>[2x]MAHHHHHHMVSWFKKIFKKEEKES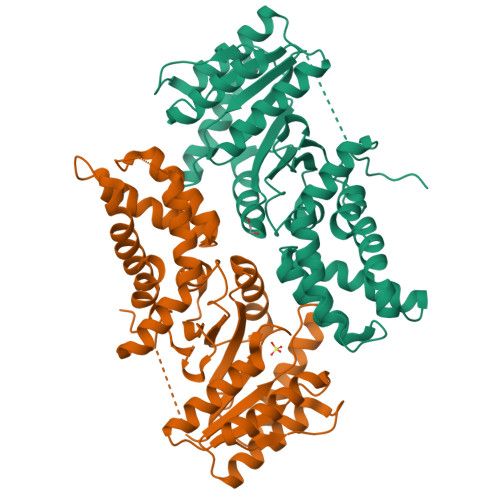LDKGLEKSSQSFFDKVSRAVVGKSKVDDEVLDDLEEVLIASDVGVETTVKIIRRIEERVARDKYVNVAELNNILREEISGLLLENPHAGTQNIDKTKKPYVIMVVGVNGVGKTTTIGKLAHQFKSEGLKVVLGAADTFRAAAVDQLVIWSERVGVPIVKQAMGSDPASVAFDTVQSAVSQDADVVIIDTAGRLHNKVNLMNELSKIKRVMQKVVPDAPHEVLLVLDGSTGQNAFEQAKQFTAATEVTALAVTKLDGTARGGVVIGISDQFQVPVKYIGVGEKMQDLQLFNGTEFVDSFFKKREEN>GAMGSGASFVQIKFDDLQFFENCGGGSFGSV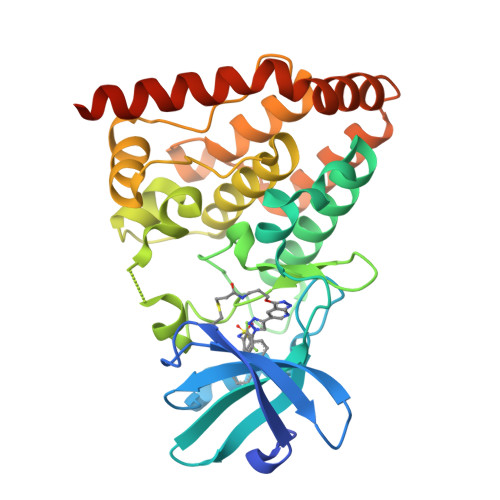YRAKWISQDKEVAVKKLLKIEKEAEILSVLSHRNIIQFYGVILEPPNYGIVTEYASLGSLYDYINSNRSEEMDMDHIMTWATDVAKGMHYLHMEAPVKVIHRDLKSRNVVIAADGVLKICDFGASRFHNHTTHMSLVGTFPWMAPEVIQSLPVSETCDTYSYGVVLWEMLTREVPFKGLEGLQVAWLVVEKNERLTIPSSCPRSFAELLHQCWEADAKKRPSFKQIISILESMSNDTSLPDKCNSFLHNKAEWRCEIEATLERLKKLERDLSFKEQELK[4x]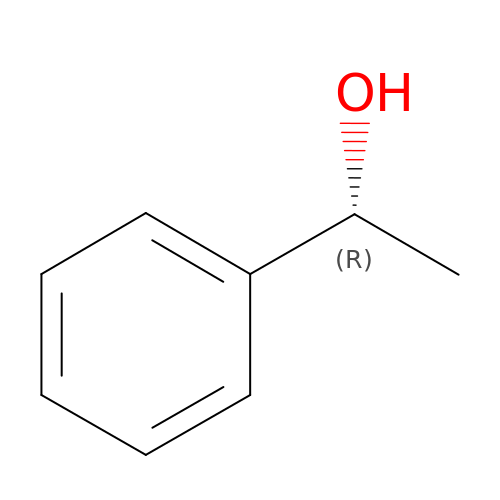(1R)-1-PHENYLETHANOL | C8 H10 O | WAPNOHKVXSQRPX-SSDOTTSWSA-N> SNASAMAQKEEGHEAAAAEAKKETDLAHVDQVETFVGKEKYYVVKGTDKKGTALYVWVPADKKAKILSKEAKEGISEDKAAKIIKDEGLVSKQKEVHLAREGNVLLWEVTYLDKEGQYSLSYVDFTTGKILKNI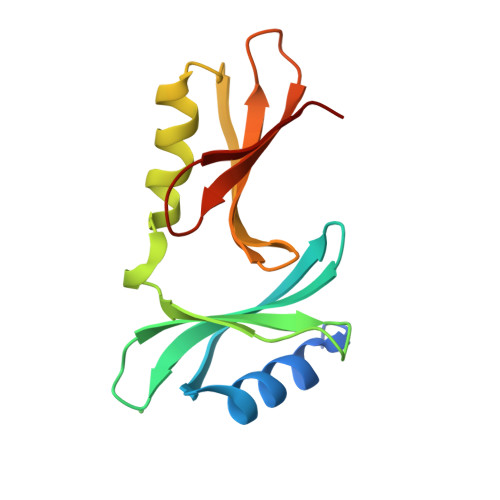TP> GSHMFGKGGLGGLMKQAQQMQEKMQKMQEEIAQLEVTGESGAGLVKITINGAHNCRRIDID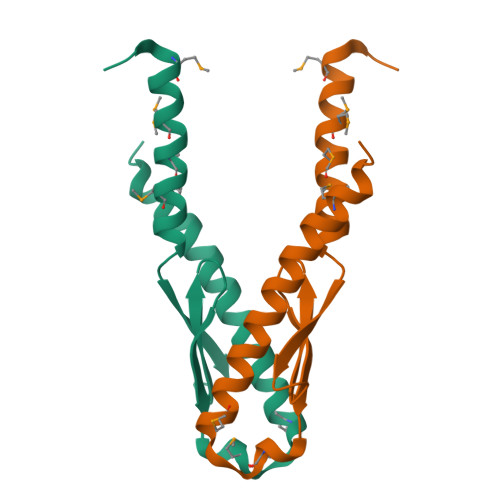PSLMEDDKEMLEDLIAAAFNDAVRRAEELQKEKMASVTAGMPLPPGMKFPF>EPETALLVAFVAYYTALIALIFAILATRRLC[9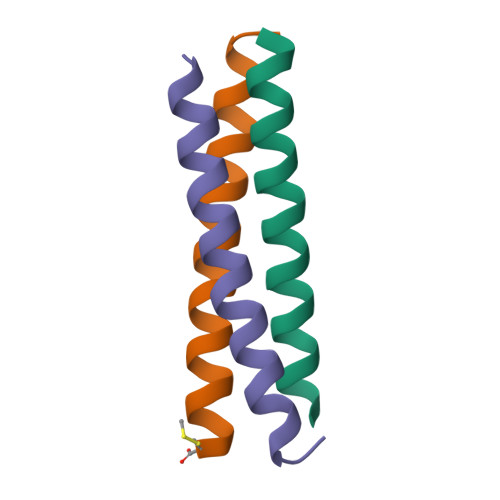x]>[3x]MPLGLLWLGLALLGALHAQAQDSTSDLIPAPPLSKVPLQQNFQDNQFQGKWYVVGLAGNAILREDKDPQKMYATIYELKEDKSYNVTSVL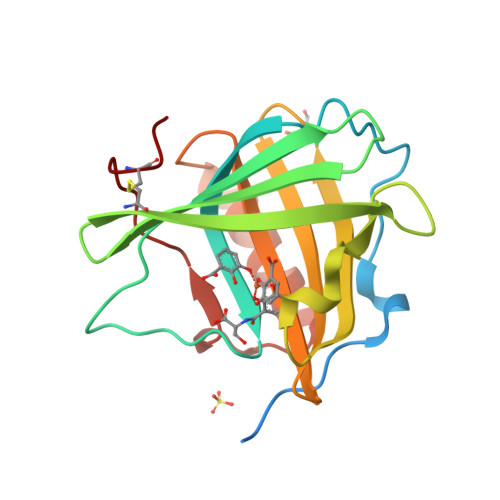FRKKKCDYAIATFVPGSQPGEFTLGNIKSYPGLTSYLVRVVSTNYNQHAMVFFKKVSQNREYFKITLYGRTKELTSELKENFIRFSKSLGLPENHIVFPVPIDQCIDG> GGGCGUAACCUCCAUCCGAGUUGCAAGAGAGGGAAA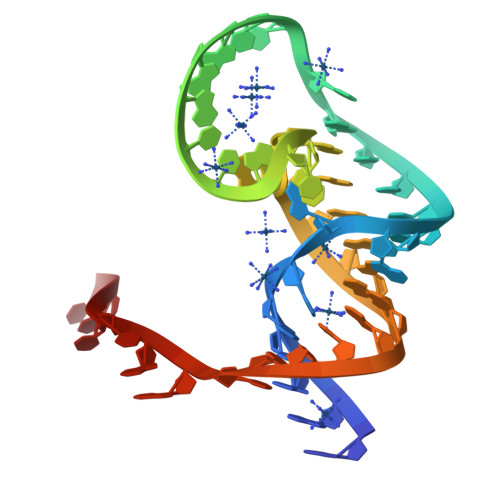CGCAGUCUC>ANAKRIEGLDSNVWVEFTKLAADPSVVNLGQGFPDISPPSYVKEELSKAAFIDNMNQYTRGFGHPALVKALSCLYGKIYQRQIDPNEEILVAVGAYGSLFNSIQGLVDPGDEVIIMVPFYDCYEPMVRMAGAVPVFIPLRSKPTDGMKWTSSDWTFDPRELESKFSSKTKAIILNTPHNPLGKVYTRQELQVIADLCVKHDTLCISDEVYEWLVYTGHTHVKIATLPGMWERTITIGSAGKTFSVTGWKLGWSIGPAHLIKHLQTVQQNSFYTCATPLQAALAEAFWIDIKRMDDPECYFNSLPKELEVKRDRMVRLLNSVGLKPIVPDGGYFIIADVSSLGADLSDMNSDEPYDYKFVKWMTKHKKLTAIPVSAFCDSKSKPHFEKLVRFCFIKKDSTLDAAEEIFRA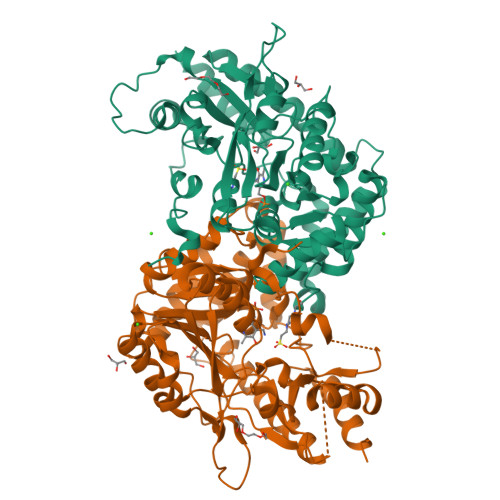WN[2x]[(2R)-1-(4-amino-2-oxo-pyrimidin-1-yl)-3-hydroxy-propan-2-yl]oxymethylphosphonic acid | 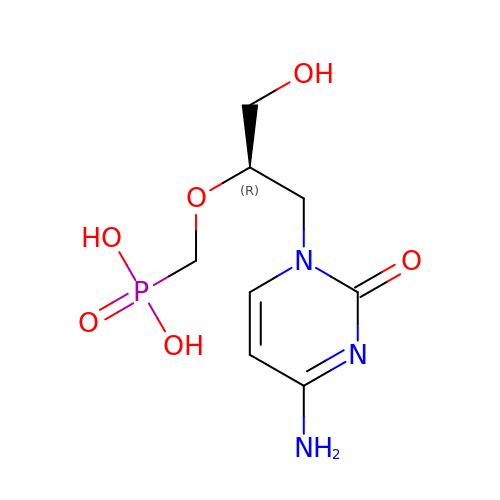C8 H14 N3 O6 P | VWFCHDSQECPREK-ZCFIWIBFSA-N>MGSSHHHHHHSSGLVPRGSMTDTGTGTGNTETDIGIIGSGISGLQLALRLQQLGVPVTLYSAQTAEELGSGRPRNFPARFAPTQAREDSLGVHAWQFDDARVHSCAITIHGEGAPLEFAGALAPPSSVVDFRLYLPHLLTEFARRGGNVRIGPVVVDEVARRHDLVVVANGDRSMRELFPRDPERSPHTTPQRILCSGFYHGIREDVPHELDIHFLPGIGEILRIPFLSRLGPAHVLAFEAVPGGPLEAPAHLDAAADPAGFHREVLRLLAAYAPSLRERVDTARFGLVAPGELAQGGVTPTVRRGWARLADGTCALAIGDAWITNDPLTAQGANLGSHTAFALADLIASATGPLDEAFCRDASARLWDHARHVVEWSNA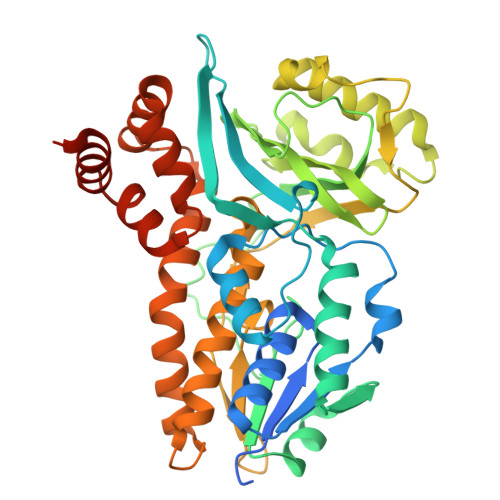FLAPPPPHVMELFGRAAGDKQIADAFVGRFHDPVAMWAVLSSPEGVDSFVRSCTEGGRHVTDVAHG[7x]> GAMEDENILRNAVNLQVL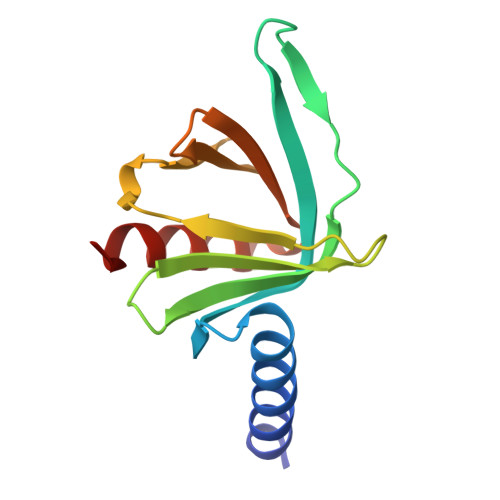KFHYPEIESIIDIASHVAVYQFDVGSQKWLKTSIEGTFFLVKDQRARVGYVILNRNSPENLYLFINHPSNVHLVDRYLIHRTENQHVVGLWMFDPNDMSRIFNIVKESLLR> MDSQGLKTAVAIFLATTFSATSYQACSAGPDTAPSLTVQQSNALPTWWKQAVFYQVYPRSFKDTNGDGIGDLNGIIENLDYLKKLGIDAIWINPHYDSPNTDNGYDIRDYRKIMKEYGTMEDFDRLISEMKKRNMRLMIDIVINHTSDQHAWFVQSKSGKNNPYRDYYFWRDGKDGHAPNNYPSFFGGSAWEKDDKSGQYYLHYFAKQQPDLNWDNPKVRQDLYDMLRFWLDKGVSGLRFDTVATYSKIPNFPDLSQQQLKNFAEEYTKGPKIHDYVNEMNREVLSHYDIATAGEIFGVPLDKSIKFFDRRRNELNIAFTFDLIRLDRDADERWRRKDWTLSQFRKIVDKVDQTAGEYGWNAFFLDNHDNPRAVSHFGDDRPQWREHAAKALATLTLTQRATPFIYQGSELGMTNYPFKKIDDFDDVEVKGFWQDYVETGKVKAEEFLQNVRQTSRDNSRTPFQWDASKNAGFTSGTPWLKINPNYKEINSADQINNPNSVF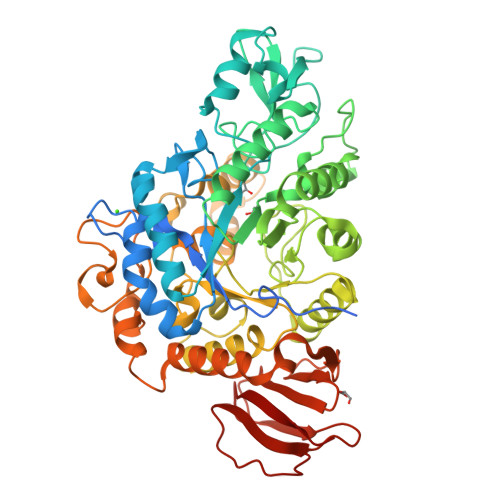NYYRKLINIRHDIPALTYGSYIDLDPDNNSVYAYTRTLGAEKYLVVINFKEEVMHYTLPGDLSINKVITENNSHTIVNKNDRQLRLEPWQSGIYKLNP> MGDLSCPEGLEELLSAPPPDLGAQRR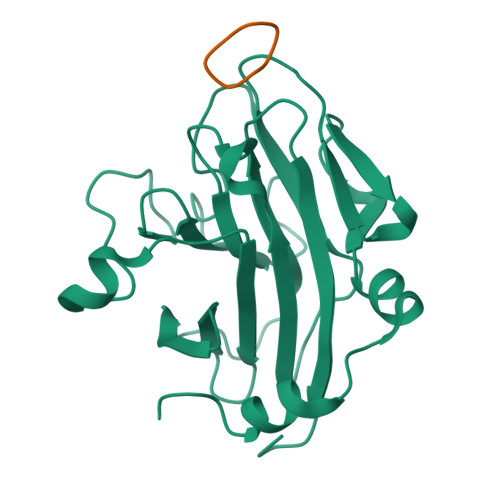HGWNPKDCSENIEVKEGGLYFERRPVAQSTDGARGKRGYSRGLHAWEISWPLEQRGTHAVVGVATALAPLQTDHYAALLGSNSESWGWDIGRGKLYHQSKGPGAPQYPAGTQGEQLEVPERLLVVLDMEEGTLGYAIGGTYLGPAFRGLKGRTLYPAVSAVWGQCQVRIRYLGERGSHHHHHH;> RGDINNN> GAMGRGNYDAFR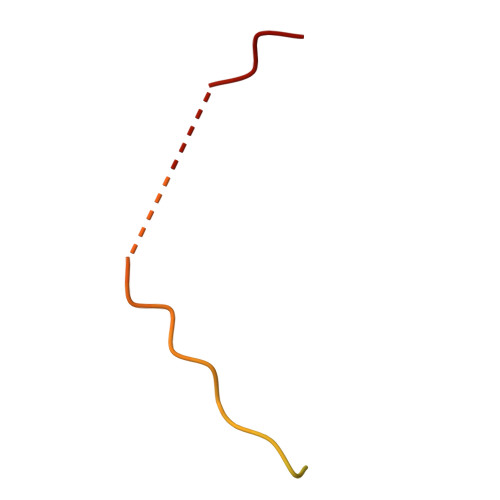GQGGYPGKPRNRMVRGDPRAIVEYRDLDAPDDVDFF>[2x]SMGKEKSK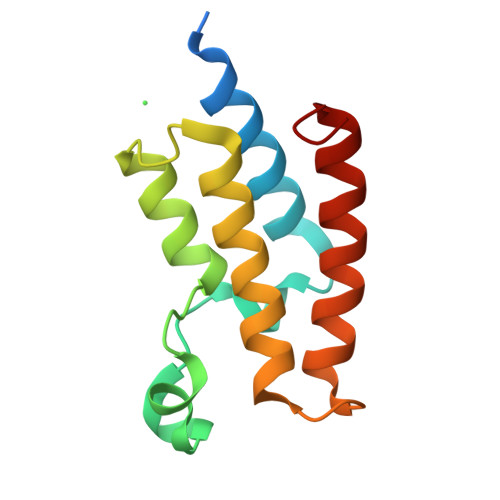EPRDPDQLYSTLKSILQQVKSHQSAWPFMEPVKRTEAPGYYEVIRFPMDLKTMSERLKNRYYVSKKLFMADLQRVFTNCKEYNPPESEYYKCANILEKFFFSKIKEAGLID> XSKYSLAPVAKELQSLLGKDVTFLNDCVGPEVEAAVKASAPGSVILLENLRYHIEEEGSRKVDGQKVKASKEDVQKFRHELSSLADVYINDAFGTAHRAHSSMVGFDLPQRAAGFLLEKELKYFGKALENPTRPFLAILGGAKVADKIQLIDNLLDKVDSIIIGGGMAFTFKKVLENTEIGDSIFDKAGAEIVPKLMEKAKAKGVEVVLPVDFI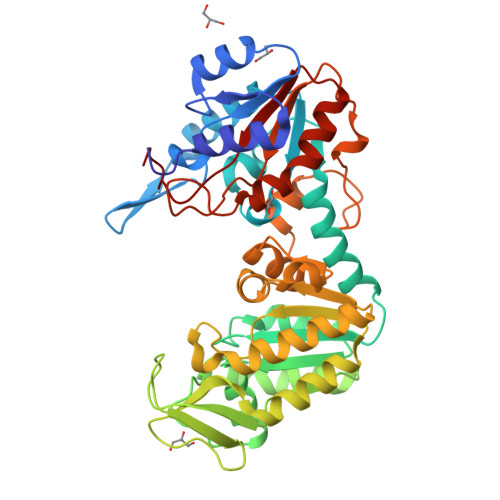IADAFSADANTKTVTDKEGIPAGWQGLDNGPESRKLFAATVAKAKTIVWNGPPGVFEFEKFAAGTKALLDEVVKSSAAGNTVIIGGGDTATVAKKYGVTDKISHVSTGGGASLELLEGKELPGVAFLSEKKSLSSKLSVQDLDLKDKRVFIRVDFNVPLDGKKITSNQRIVAALPTIKYVLEHHPRYVVLASHLGRPNGERN> GNN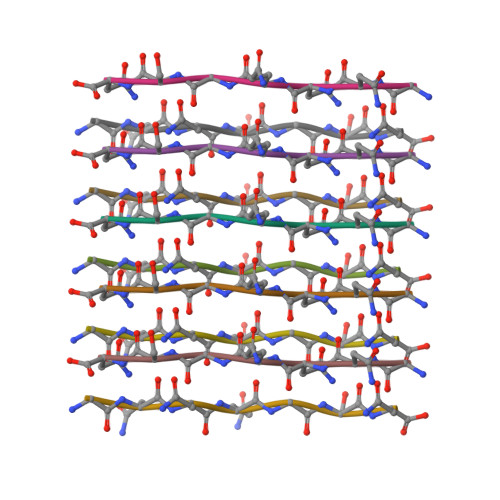QGSN>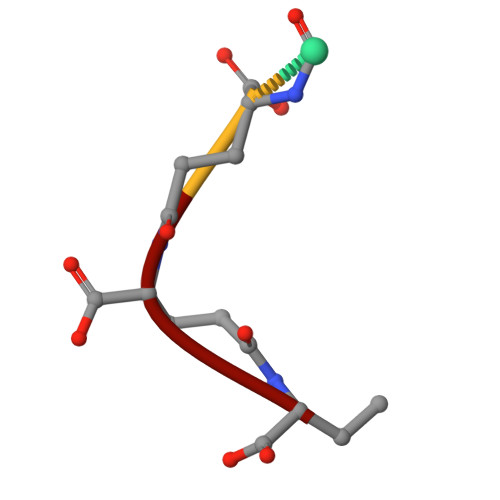 EEEE>MQLVLAAKYIGAGISTIGLLGAGIGIAIVFAALINGVSRNPSIKDTVFPMAILGFALSEATGLFCLMVSFLLLFGV[20x];>[2x]MPQLVPFYFMNQLTYGFLLMITLLILFSQFFLPMILRLYVSRLFISKL;>[2x]SPLDQFEIRTLFGLQSSFIDLSCLNLTTFSLYTIIVLLVITSLYTLTNNNNKIIGSRWLISQEAIYDTIMNMTKGQIGGKNWGLYFPMIFTLFMFIFIANLISMIPYSFALSAHLVFIISLSIVIWLGNTILGLYKHGWVFFSLFVPAGTPLPLVPLLVIIETLSYFARAISLGLRLGSNILAGHLLMVILAGLTFNFMLINLFTLVFGFVPLAMILAIMMLEFAIGIIQGYVWAILTASYLKDAVYLH;>[2x]MSSTPEKQTDPKAKANSIINAIPGNNILTKTGVLGTSAAAVIYAISNELYVINDESILLLTFLGFTGLVAKYLAPAYKDFADARMKKVSDVLNASRNKHVEAVKDRIDSVSQLQNVAETTKVLFDVSKETVELESEAFELKQKVELAHEAKAVLDSWVRYEASLRQLEQRQLAKSVISRVQSELGNPKFQEKVLQQSISEIEQLLSKLK;>SLAKSAANKLDWAKVIS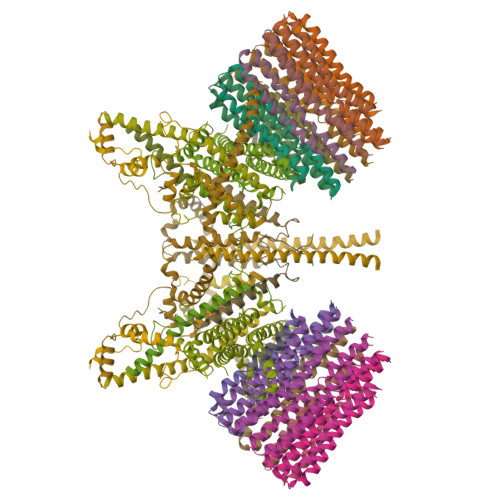SLRITGSTATQLSSFKKRNDEARRQLLELQSQPTEVDFSHYRSVLKNTSVIDKIESYVKQYKPVKIDASKQLQVIESFEKHAMTNAKETESLVSKELKDLQSTLDNIQSARPFDELTVDDLTKIKPEIDAKVEEMVKKGKWDVPGYKDRFGNLNVM[2x];>[2x]VSTLIPPKVVSSKNIGSAPNAKRIANVVHFYKSLPQGPAPAIKANTRLARYKAKYFDGDNASGKPLWHFALGIIAFGYSMEYYFHLRHHKGAEEH;>MLKRFPTPILKVYWPFFVAGAAVYYGMSKAADLSSNTKEFINDPRNPRFAKGGKFVEVD[2x];>MGAAYHFMGKAIPPHQLAIGTLGLLGLLVVPNPFKSAKPKTVDIKTDNKDEEKFIENYLKKHSEKQDA[2x]>MKILITGGAGFIGSAVVRHIIKNTQDTVVNIDKLTYAGNLESLSDISESNRYNFEHADICDSAEITRIFEQYQPDAVMHLAAESHVDRSITGPAAFIETNIVGTYALLEVARKYWSALGEDKKNNFRFHHISTDEVYGDLPHPDEVENSVTLPLFTETTAYAPSSPYSASKASSDHLVRAWRRTYGLPTIVTNCSNNYGPYHFPEKLIPLVILNALEGKPLPIYGKGDQIRDWLYVEDHARALHMVVTEGKAGETYNIGGHNEKKNLDVVFTICDLLDEIVPKATSYREQITYVADR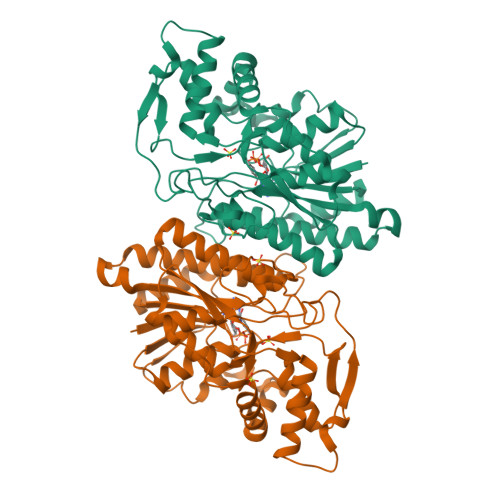PGHDRRYAIDAGKISRELGWKPLETFESGIRKTVEWYLANTQWVNNVKSGAYQSWIEQNYEGRQ[4x]During activation of a pentameric ligand-gated ion channel (pLGIC), the binding of agonists promotes the opening of a selective ion conduction pore at a distance of more than 50 Å away from the binding sites. Each subunit consists of a predominantly β-stranded extracellular domain and an α-helical transmembrane pore, which interact via an extended interface. Whereas ELIC forms a cation-selective channel with high conductance that is activated with high efficacy by the primary amines cysteamine, propylamine, and GABA, the cation-selective GLIC is activated by protons and inhibited by bulky positively charged compounds that also act as open channel blockers of the nAChR. Our study has identified a cluster of interacting residues located at the β1-β2 turn, the β6-β7 loop and the pre-M1 region of the extracellular domain, and the M2-M3 loop of the pore that exert a strong influence on channel function.

At the tip of the GLIC β1-β2 turn, immediately adjacent to Asp31, Lys32 interacts with a strictly conserved proline in the M2-M3 loop (Pro254 in ELIC and Pro246 in GLIC). We thus suspected that this interaction might play an important role for the relay of conformational changes from the extracellular domain to the pore. Mutations of the conserved proline in the M2-M3 loop to alanine (P246A in GLIC and P254A in ELIC) resulted in channels that, apart from a small shift in the EC50 in the case of GLIC, show robust activation with similar properties as WT. In line with the comparably small effect in functional experiments, the crystal structure of the GLIC mutant P246A is virtually identical to WT. Contrary to our previous expectation, conformational changes appear not to be predominantly transduced via an interaction of the tip of the β1-β2 turn to a conserved proline in the M2-M3 loop of the pore domain (Pro254 in ELIC and Pro246 in GLIC), as mutations of this residue to alanine and glycine still permit channel activation. Critical interactions involve residues of the M2-M3 loop, the pre-M1 region and the β1-β2 turn that all contact the β6-β7 loop, whereas a direct interaction between the β1-β2 turn and the M2-M3 loop appears expendable.

>[5x]QDMVSPPPPIADEPLTVNTGIYLIECYSLDDKAETFKVNAFLSLSWKDRRLAFDPVRSGVRVKTYEPEAIWIPEIRFVNVENARDADVVDISVSPDGTVQYLERFSARVLSPLDFRRYPFDSQTLHIYLIVRSVDTRNIVLAVDLEKVGKNDDVFLTGWDIESFTAVVKPANFALEDRLESKLDYQLRISRQYFSYIPNIILPMLFILFISWTAFWSTSYEANVTLVVSTLIAHIAFNILVETNLAKTPYMTYTGAIIFMIYLFYFVAVIEVTVQHYLKVESQPARAASITRASRIAFPVVFLLANIILAFLFFGF> MGSHHHHHHSGSMSIASIDRVAAQGHWRSRPLAEKSLIGLGFLALAVTVPPFPGAVLVTVAILAFTFLGARVPLRFWASVAVLPLGFLTTGAAVLLIQIGPEGIGLAPDGPAKAAALVMRATAATCCLLFLATTTPAADLLSGLRRWRVPAELIEIALLTYRFVFILAEEAAAMTTAQRARLGHATRRRWLRSTAQVIAALLPRALTRARRLETGLGARNWQGEMRVLSTRPPASARVLGLI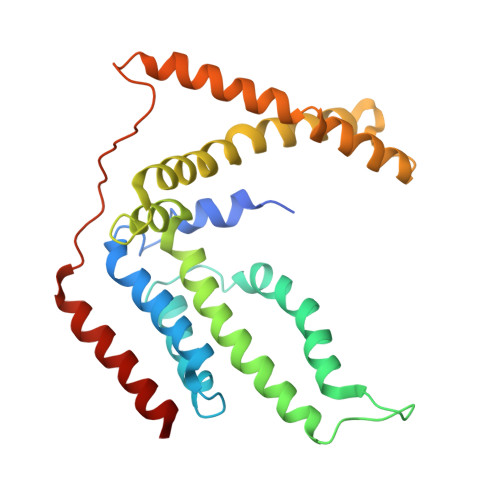LTLQAAILAAGVLL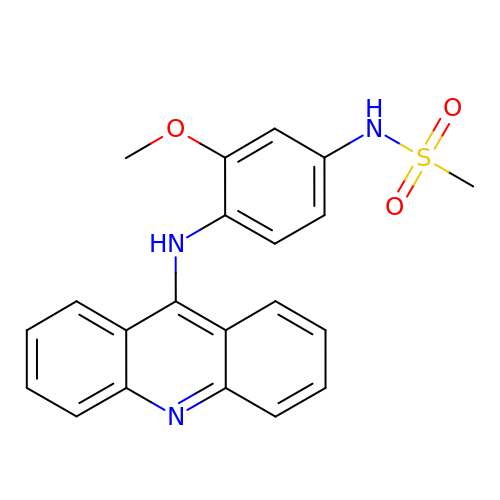N-[4-(acridin-9-ylamino)-3-methoxyphenyl]methanesulfonamide | C21 H19 N3 O3 S | XCPGHVQEEXUHNC-UHFFFAOYSA-N>MPPYTVVYFPVRGRCAALRMLLADQGQSWKEEVVTVETWQEGSLKASCLYGQLPKFQDGDLTLYQSNTILRHLGRTLGLYGKDQQEAALVDMVNDGVEDLRCKYISLIYTNYEAGKDDYVKALPGQLKPFETLLSQNQGGKTFIVGDQISFADYNLLDLLLIHEVLAPGCLDAFPLLSAYVGRLSARPKLKAFLASPEYVNLPINGNGKQ[2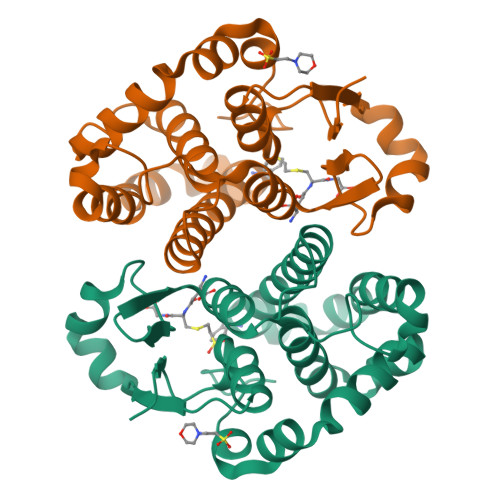x]>NSLEIDSLARFAVEEHNKKQNALLEFGRVVSAQ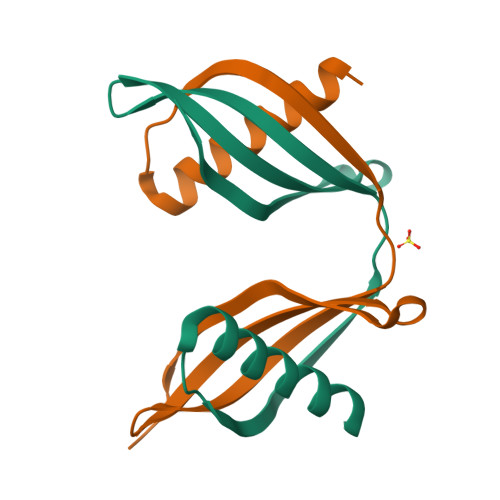QQVVSGTLYTITLEAKDGGQKKVYEAKVWEKPWLNFKELQEFKHVGDAPA[2x]8-bromo-4-oxo-1,4-dihydroquinoline-3-carboxylic acid | C10 H6 Br N O3 | 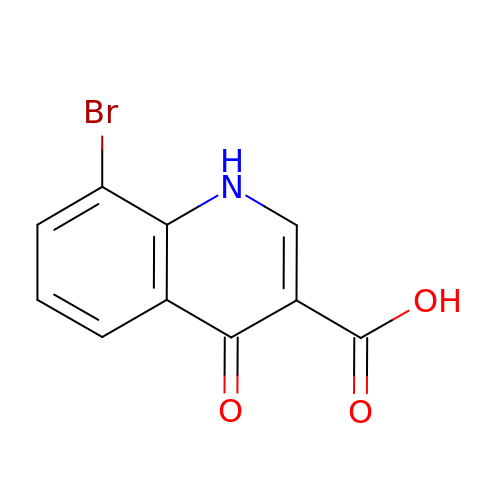NKUGXZLINWIUOR-UHFFFAOYSA-N> RVLFSQAQVYELERRFKQQRYLSAPERDQLASV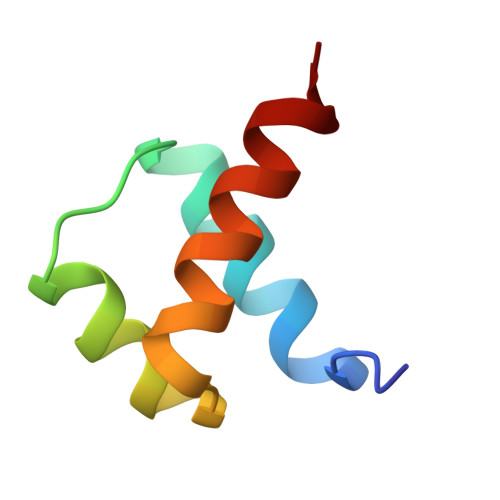LKLTSTQVKIWFQNRRYKSK> GSTPDQQTLLHFIMDSYNKQRMPQEITNKILKEEFSAEENFLILTEMATNHVQVLVEFTKKLPGFQTLDHEDQIALLKGSAVEAMFLR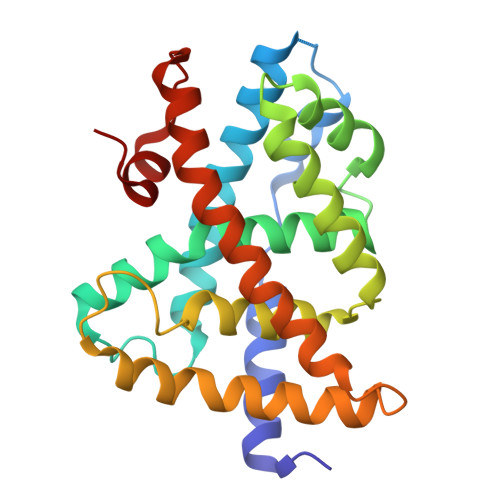SAEIFNKKLPSGHSDLLEERIRNSGISDEYITPMFSFYKSIGELKMTQEEYALLTAIVILSPDRQYIKDREAVEKLQEPLLDVLQKLCKIHQPENPQHFAELLGRLTELRTFNHHHAEMLMSWRVNDHKFTPLLEEIWDVQ> GSLHMIDYKEIEVEEVVGRGAFGVVCKAKWRAKDVAIKQIESESERKAFIVELRQLSRVNHPNIVKLYGACLNPVCLVMEYAEGGSLYNVLHGAEPLPYYTAAHAMSWCLQCSQGVAYLHSMQPKALIHRDLKPPNLLLVAGGTVLKICDFGTACDIQTHMTNNKGSAAWMAPEVFEGSNYSEKCDVFSWGIILWEVITRRKPFDEIGGPAFRIMWAVHNGTRPPLIKNLPKPIESLMTRCWSKDPSQRPSMEEIVKIMTHLMRYFPGADEPL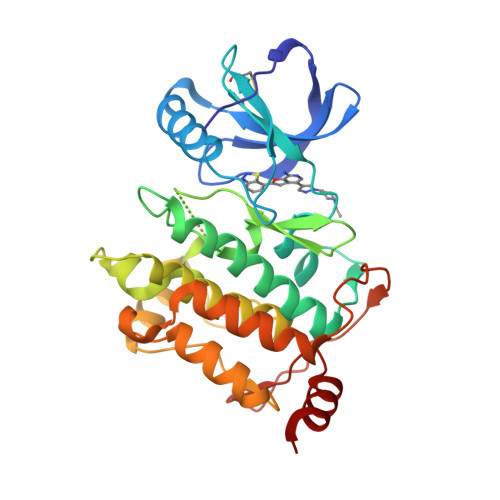QYPCQHSLPPGEDGRVEPYVDFAEFYRLWSVDHG>GHMKCPVCHQGEMVSGIKDIPYTFRGRKTVLKGIHGLYCVHCEESIMNKEESDAFMAQVKAFR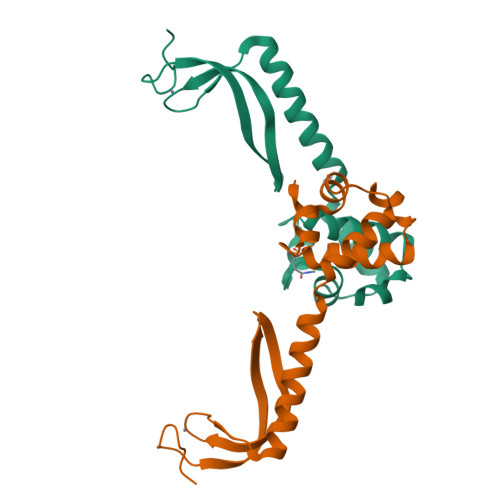ASVNAETVAPEFIVKVRKKLSLTQKEASEIFGGGVNAFSRYEKGNAQPHPSTIKLLRVLDKHPELLNEIR[2x]>MEFRQLKYFIAV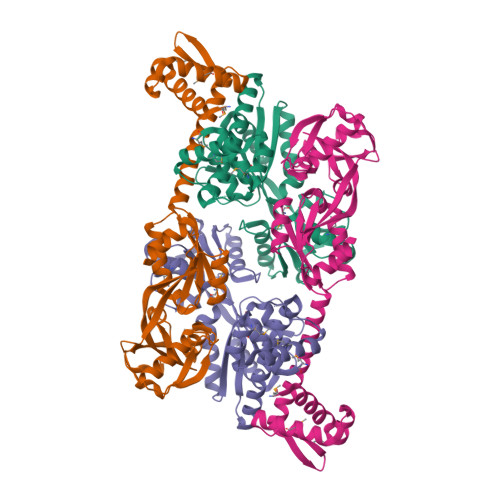AEAGNMAAAAKRLHVSQPPITRQMQALEADLGVVLLERSHRGIELTAAGHAFLEDARRILELAGRSGDRSRAAARGDVGELSVAYFGTPIYRSLPLLLRAFLTSTPTATVSLTHMTKDEQVEGLLAGTIHVGFSRFFPRHPGIEIVNIAQEDLYLAVHRSQSGKFGKTCKLADLRAVELTLFPRGGRPSFADEVIGLFKHAGIEPRIARVVEDATAALALTMAGAASSIVPASVAAIRWPDIAFARIVGTRVKVPISCIFRKEKQPPILARFVEHVRRSAKD[2x]> PKVSVLITVTGVDQPGVTATLFEVLSRHGVELLNVEQVVIRHRLTLGVLVCCPADVADGPALRHDVEAAIRKVGLDVSIERSDDVPIIREPSTHTIFVLGRPITAAAFGAVAREVAA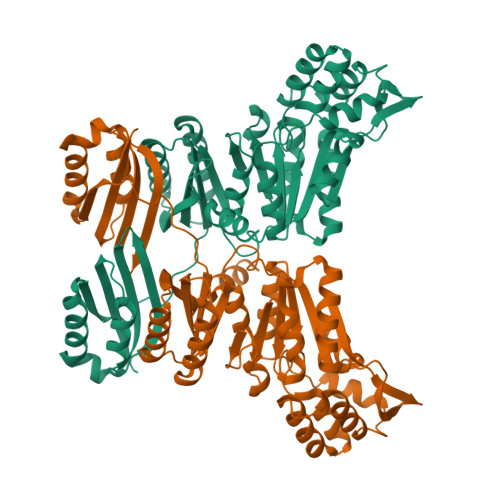LGVNIDLIRGVSDYPVIGLELRVSVPPGADGALRTALNRVSSEEHVDVAVEDYTLERRAKRLIVFDVDSTLVQGEVIEMLAAKAGAEGQVAAITDAAMRGELDFAQSLQQRVATLAGLPATVIDEVAGQLELMPGARTTLRTLRRLGYACGVVSGGFRRIIEPLAEELMLDYVAANELEIVDGTLTGRVVGPIIDRAGKATALREFAQRAGVPMAQTVAVGNGANDIDMLAAAGLGIAFNAKPALREVADASLSHPYLDTVLFLLGVTRGEIEAADAID> GGCUUAUCAAGAGAGGU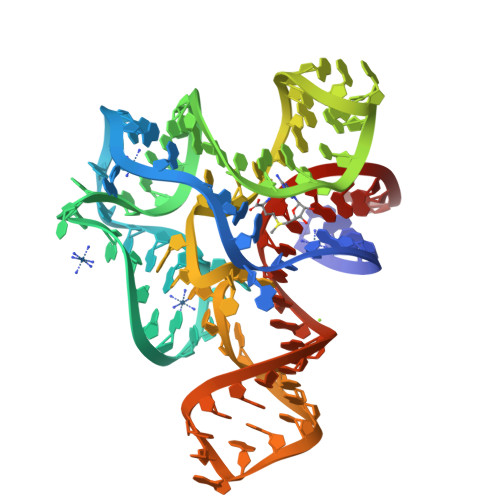GGAGGGACUGGCCCGAUGAAACCCGGCAACCAGAAAUGGUGCCAAUUCCUGCAGCGGAAACGUUGAAAGAUGAGCCA>MATVQPIVNSHLSELDEDVFHHFGFTTKSFDFKEKFGDV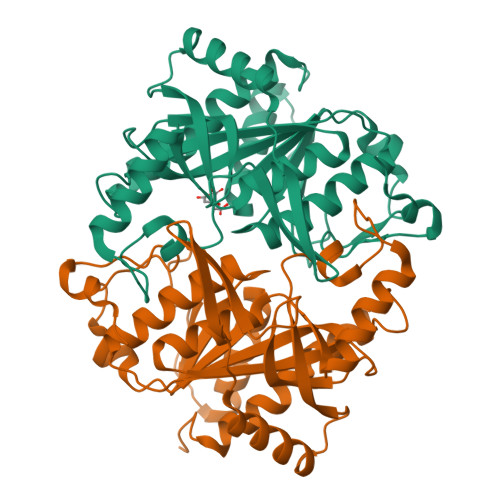KFVCVCGSSGRIHNFAISMAKLAGLALPVENIAGSHARFVLYKVDHILFADHGIGIPSTLILMHEVTKLLYYAGCKDVLFIRLGTSDGLGVKPGTIVLSDRCVNTKLEPYNELCILGKPVRRQTKVDSNAVNELKKLSENLSLKCSVVVGGTITANDFYEELGRLNGSICTFSKEEKLAFLQSVYDHGIRNMEMEGAAITSHCNLTGHRAILVCVTVVNRLETDEVTTSTDEFKLFEQLPGQLVGEYLKRNNGIIVR[3x]> MNKHSGIDFKQLNFLTKLNENHSGEWWKGRWQGNDIVVKVLKVRDWSTRKSRDFNEECPRLRIFSHPNVLPVLGACQSPPAPHPTLITHWMPYGSLYNVLHE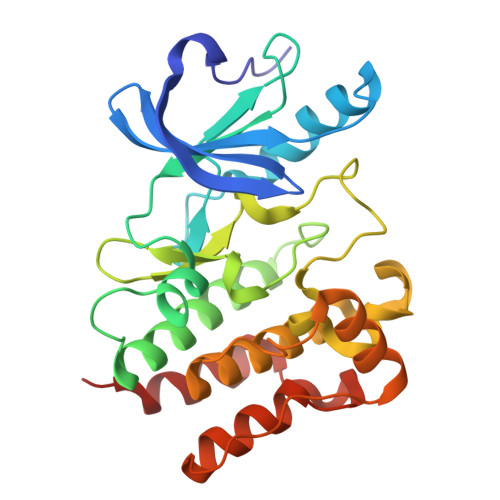GTNFVVDQSQAVKFALDMARGMAFLHTLEPLIPRHALNSRSVMIDEDMTARISMADVKFSFQSPGRMYAPAWVAPEALQKKPEDTNRRSADMWSFAVLLWELVTREVPFADLSNMEIGMKVALEGLRPTIPPGISPHVSKLMKICMNEDPAKRPKFDMIVPILEKMQDK> RPQKAIAVMTSGGDAPGMNSNVRAIVRSAIFKGCRAFVVMEGYEGLVRGGPEYIKEFHWEDVRGWSAEGGTNIGTARCMEFKKREGRLLGAQHLIEAGVDALIVCGGDGSLTGADLFRSEWPSLIEELLKTNRISNEQYERMKHLNICGTVGSIDNDMSTTDATIGAYSALDRICKAIDYVEATANSHSRAFVVEVMGRNCGWLALLAGIATSADYIFIPEKPATSSEWQDQMCDIVSKHRSRGKRTTIVVVAEGAIAADLTPISPSDVHKVLVDRLGLDTRITTLGHVQRGGTAVAYDRILATLQGLEAVNAVLESTPDTPSPLIAVNENKIVRKPLMESVKLTKAVAEAIQAKDFKRAMSLRDTEFIEHLNNFMAINSADHNEPKLPKDKRLKIAIVNVGAPAGGINSAVYSMATYCMSQGHRPYAIYNGWSGLARHESVRSLNWKDMLGWQSRGGSEIGTNRVTPEEADLGMIAYYFQKYEFDGLIIVGGFEAFESLHQLERARESYPAFRIPMVLIPATLSNNVPGTEYSLGSDTALNALMEYCDVVKQSASSTRGRAFVVDCQGGNSGYLATYASLAVGAQVSYVPEEGISLEQLSEDIEYLAQSFEKAEGRGR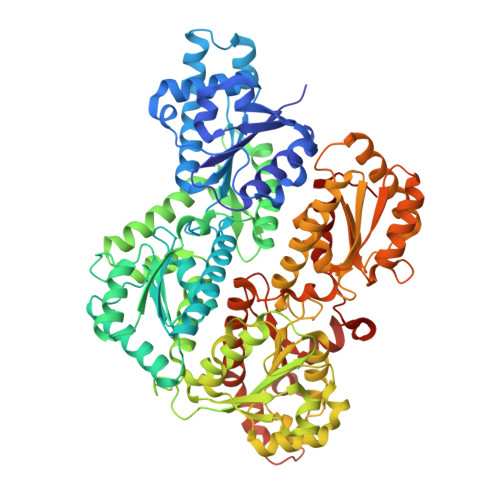FGKLILKSTNASKALSATKLAEVITAEADGRFDAKPAYPGHVQQGGLPSPIDRTRATRMAIKAVGFIKDNQAAIAEARAAEENFNADDKTISDTAAVVGVKGSHVVYNSIRQLYDYETEVSMRMPKVIHWQATRLIADHLVGRKRVD>[4x]TASGINDGSGIVLGKDRDGG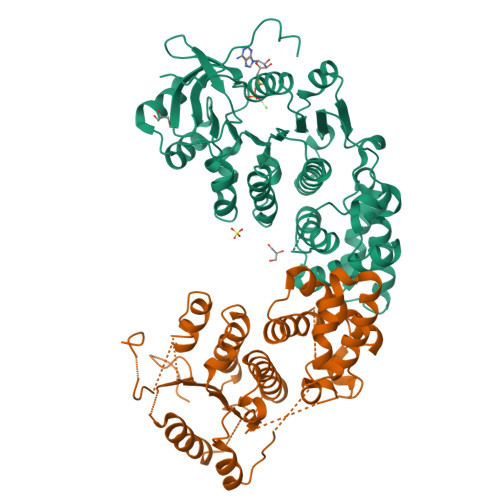LVLVDIWKRGGDRTNSNWTILAKPGAGKSFTAKMLLLREYMQGSRVIIIDPEREYKEMCRKLGGVWINCTGGEGKINPLQVRLRPVEEEDEENAVFQSPLALHIQTLRTFFSLYLRDLTDTEKAALEDALVEVYKEAGITWDTDPRGVPNDKWPTVKELYEYCVKKAEENPETYGRLSVLLKRAAEGADSYLWAGPTAVEADSDFIVFDVHDLQNAEDQVKRAQYFNVLSFAWNILERDRRERTVLVVDEAWMLVDPQTPQAIAFLRDTSKRIRKYNGSLIVISQNVIDFLAPEVQRYGQALLDNPTYKLLLAQGEKDLEAITTLMNLSEAEHDLLVNAKRGEGLFVAGTQRIHIKIEAAPYEMQYLTGGGN>DYKDDDDKLHSQANLMRLKSDLFNRSPMYPGPTKDDPLTVTLGFTLQDIVKADSSTNEVDLVYWEQQRWKLNSLMWDPNEYGNITDFRTSAADIWTPDITAYSSTRPVQVLSPQIAVVTHDGSVMFIPAQRLSFMCDPTG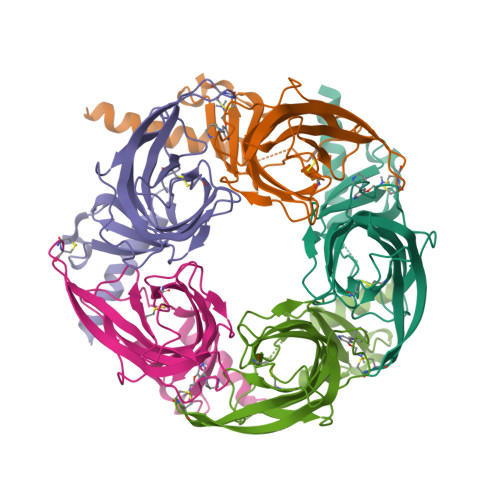VDSEEGATCAVKFGSWVYSGFEIDLKTDTDQVDLSSYYASSKYEILSATQTKHDIKYNCCEEIYTDVNLVVKFRERRAGNGFFRNLFDSR[5x]> MGEVKSVKVDNWGVFFLQKLQNFFNKTDYCDLTLQFRDNSQLKVHRLVLSACTDYFNVLEQT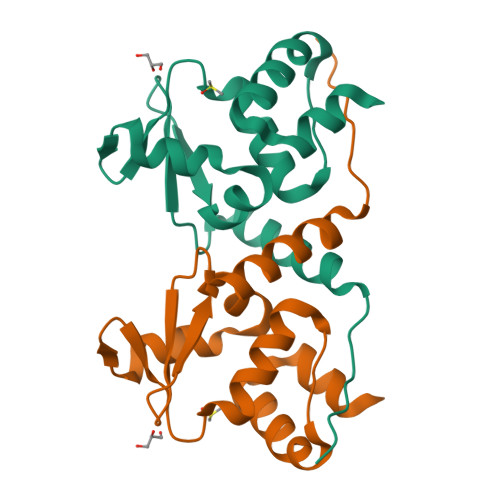CEIVDDALIMPNEFQADVVVPIVNFMYTGTLEFELKMYGKLLRTAKEMNMTVLLKLLEAHRRTMENVNRQQRHHHHHH> ANKGFLEEVRKGNLERECLEEPCSREEAFEALESLSATDAFWAKYTACESARNPREKLNECLEGNCAEGVGMNYRGNVSVTR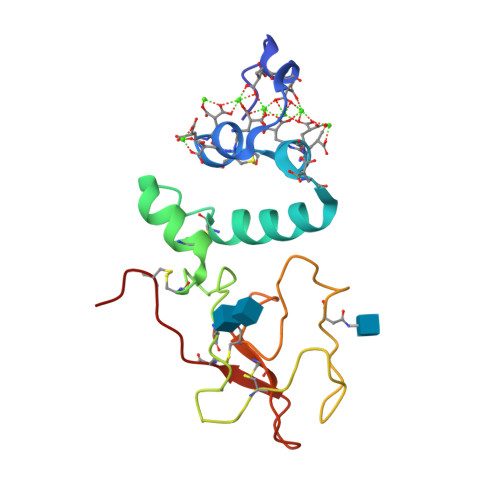SGIECQLWRSRYPHKPEINSTTHPGADLRENFCRNPDGSITGPWCYTTSPTLRREECSVPVCGQD>GPGSMSNVAVNTVFASLDNFRKGTVEIISGEARHYAFSNIFEVAQNSKPYEKVVVGLNLGYVVETLRAEGQSPWFTAAHDEFAIVMDGEVRVEFLKLDAPSKHGEGTHLAGELPVGKPMGYVLLKRGHQCLLPAGSAYRFEASRPGVILQQTIKGPLSVEKWAEICLK[2x];>MAMLESAVDSAAFADDDVQASPPHAVTGYRSFQLGAFELSRDEYFARITWPAKGETRSHLIPADIFLRAMMRDVAWGFFYGWVNFDHVIGTRNYYGKVDLYAGTFNGTLKAAGVNYTENFETPLIMATFKAILRDWTNATFDPFAAPEETGSAFGRKNGENLECIERFRIATKRMPG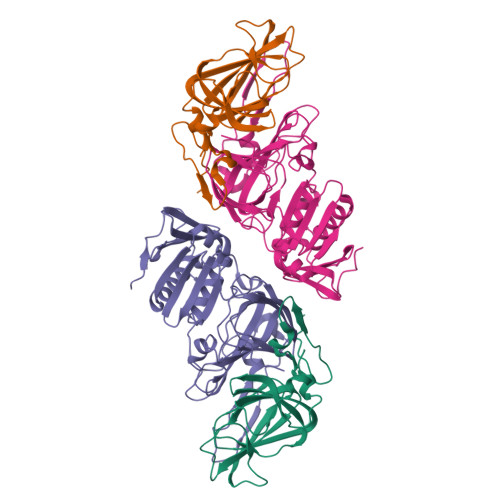LQDDSPLRNDLPVNRQFADVSQDEPEVHAAEGFEGELHAFSLFKYLSRSDVTWNPSVTSVCKASLFCPTTEEFILPVFHGNDRVEWFIQMSDEIVWDVGDKDDGNPRARITMRAGDVCAMPADIRHQGYSTKRSMLMVWENATPNLPHLYESGELKPYPIEF[2x]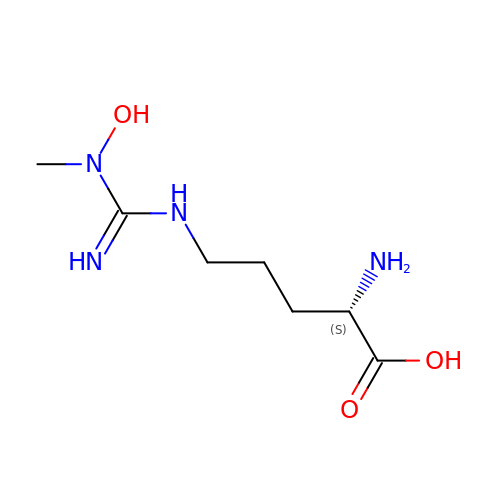N~5~-(N-hydroxy-N-methylcarbamimidoyl)-L-ornithine | C7 H16 N4 O3 | BNNZGZKJTQTHNK-YFKPBYRVSA-N> GGMLCYVTRPDAVLMEVEVEAKANGEDCLNQVCRRLGIIEVDYFGLQFTGSKGESLWLNLRNRISQQMDGLAPYRLKLRVKFFVEPHLILQEQTRHIFFLHIKEALLAGHLLCSPEQAVELSALLAQTKFGDYNQNTAKYNYEELCAKELSSATLNSIVAKHKELEGTSQASAEYQVLQIVSAMENYGIEWHSVRDSEGQKLLIGVGP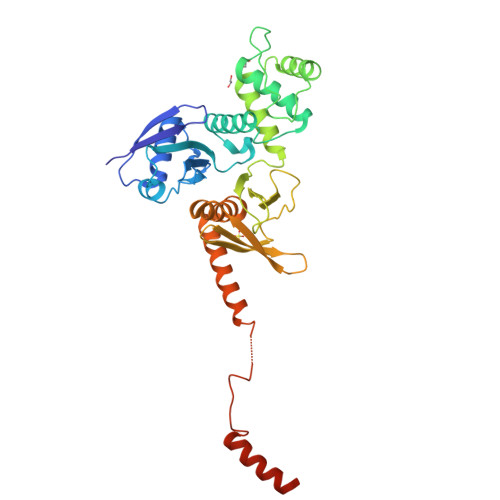EGISICKDDFSPINRIAYPVVQMATQSGKNVYLTVTKESGNSIVLLFKMISTRAASGLYRAITETHAFYRCDTVTSAVMMQYSRDLKGHLASLFLNENINLGKKYVFDIKRTSKEVYDHARRALYNAGVVDLVSRNNQ> ADTIVAVELDTYPNTDIGDPSYQHIGINIKSIRSK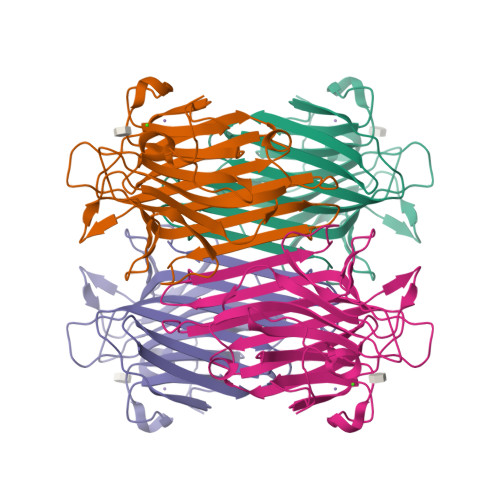ATTRWDVQNGKVGTAHISYNSVAKRLSAVVSYPGGSSATVSYDVDLNNILPEWVRVGLSASTGLYKETNTILSWSFTSKLKSNSTADAQSLHFTFNQFSQSPKDLILQGDASTDSDGNLQLTRVSNGSPQSDSVGRALYYAPVHIWDKSAVVASFDATFTFLIKSPDREIADGIAFFIANTDSSIPHGSGGRLLGLFPDAN> MNDRADFVVPDITTRKNVGLSHDANDFTLPQPLDRYSAEDHATWATLYQRQCKLLPGRACDEFLEGLERLEVDADRVPDFNKLNEKLMAATGWKIVAVPGLIPDDVFFEHLANRRF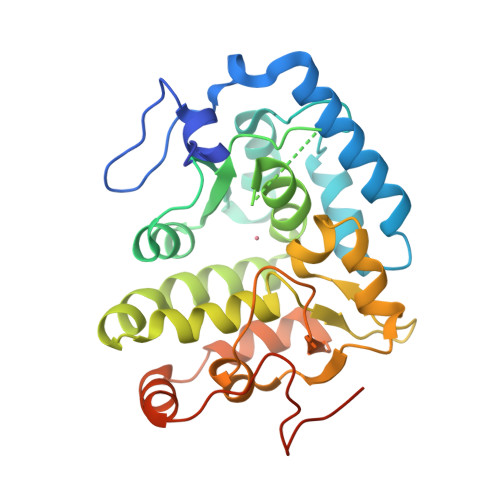PVTWWLREPHQLDYLQEPDVFHALFGHVPLLINPVFADYLEAYGKGGVKAKALGALPMLARLYWYTVEFGLINTPAGMRIYGAGILSSKSESIYCLDSASPNRVGFDLMRIMNTRYRIDTFQKTYFVIDSFKQLFDATAPDFAPLYLQLADAQPWGAGDIAPDDLVLNAGDRQGWADTEDV> MALDAFSKVVTNADAKAAYVGGADLQALKKFISEGNKRLDAVNSIVSNASCIVSDAVSGMICENPSLISPSGNCYTNRRMAACLRDGEIILRYVSYALLSGDSSVLEDRCLNG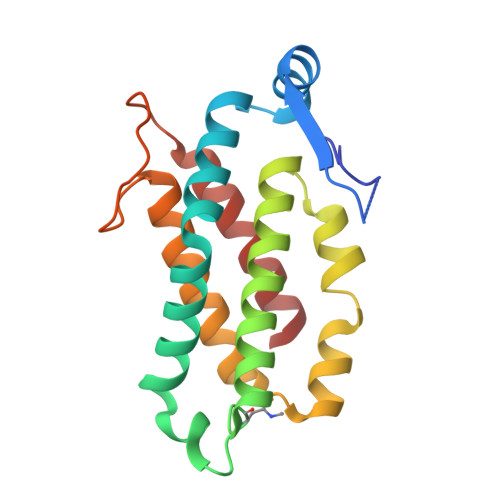LKETYSSLGVPANSNARAVSIMKACAVAFVNNTASQRKLSTPQGDCSALASEVAGYFDKVSAAIG>SMGASFVQIKFDDLQFFENCGGGSFGSVYRAKWISQDKEVAVKKLLKIEKEAEILSVLSHRNIIQFYGVILEPPNYGIVTEYASLGSLYD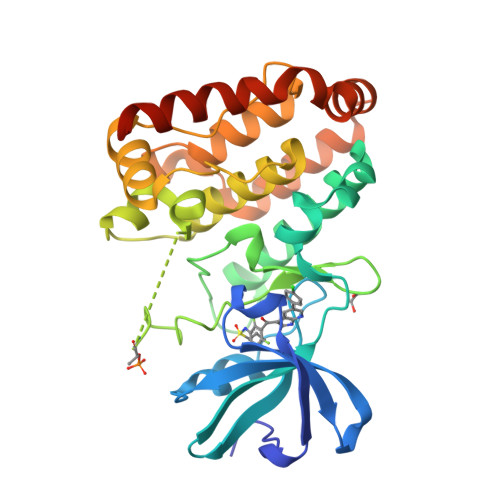YINSNRSEEMDMDHIMTWATDVAKGMHYLHMEAPVKVIHRDLKSRNVVIAADGVLKICDFGASRFHNHTTHMSLVGTFPWMAPEVIQSLPVSETCDTYSYGVVLWEMLTREVPFKGLEGLQVAWLVVEKNERLTIPSSCPRSFAELLHQCWEADAKKRPSFKQIISILESMSNDTSLPDKCNSFLHNKAEWRCEIEATLERLKKLERDLSFKEQELK[2x]>[4x]GPGSCPTHADSLNNLANIKREQGNIEEAVRLYRKALEVFPEFAAAHSNLASVLQQQGKLQEALMHYKEAIRISPTFADAYSNMGNTLKEMQDVQGALQCYTRAIQINPAFADAHSNLASIHKDSGNIPEAIASYRTALKLKPDFPDAYC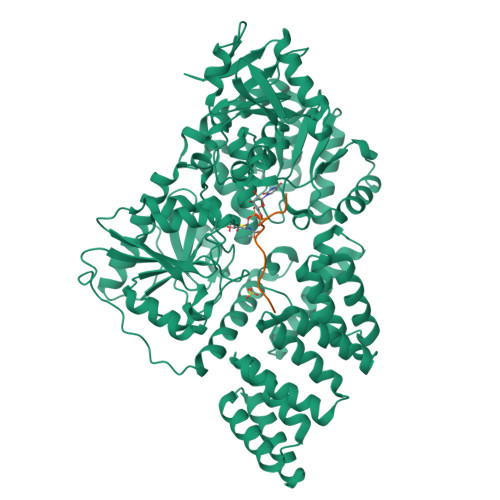NLAHCLQIVCDWTDYDERMKKLVSIVADQLEKNRLPSVHPHHSMLYPLSHGFRKAIAERHGNLCLDKINVLHKPPYEHPKDLKLSDGRLRVGYVSSDFGNHPTSHLMQSIPGMHNPDKFEVFCYALSPDDGTNFRVKVMAEANHFIDLSQIPCNGKAADRIHQDGIHILVNMNGYTKGARNELFALRPAPIQAMWLGYPGTSGALFMDYIITDQETSPAEVAEQYSEKLAYMPHTFFIGDHANMFPHLKKKAVIDFKSNGHIYDNRIVLNGIDLKAFLDSLPDVKIVKMKCPDGGDNADSSNTALNMPVIPMNTIAEAVIEMINRGQIQITINGFSISNGLATTQINNKAATGEEVPRTIIVTTRSQYGLPEDAIVYCNFNQLYKIDPSTLQMWANILKRVPNSVLWLLRFPAVGEPNIQQYAQNMGLPQNRIIFSPVAPKEEHVRRGQLADVCLDTPLCNGHTTGMDVLWAGTPMVTMPGETLASRVAASQLTCLGCLELIAKNRQEYEDIAVKLGTDLEYLKKVRGKVWKQRISSPLFNTKQYTMELERLYLQMWEHYAAGNKPDHMIKPVE;>GPVFTSRSAAG[4x]> GIPRNSRVDSDDFLWFEGIAFPTMGFRSETLRKVRDEFVIRDEDVIILTYPKSGTNWLAEILCLMHSKGDAKWIQSVPIWERSPWVESEIGYTALSETES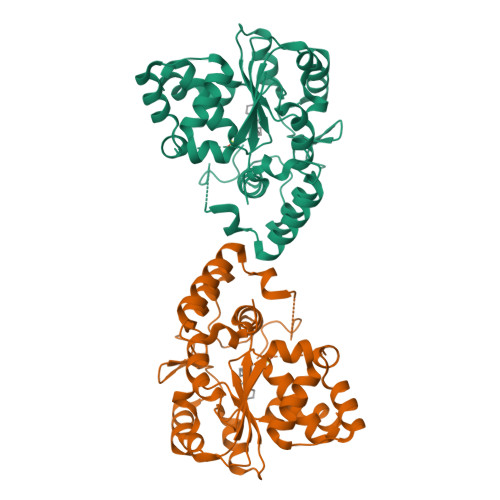PRLFSSHLPIQLFPKSFFSSKAKVIYLMRNPRDVLVSGYFFWKNMKFIKKPKSWEEYFEWFCQGTVLYGSWFDHIHGWMPMREEKNFLLLSYEELKQDTGRTIEKICQFLGKTLEPEELNLILKNSSFQSMKENKMSNYSLLSVDYVVDKTQLLRKGVSGDWKNHFTVAQAEDFDKLFQEKMADLPRELFPWE>[4x]GMTDIPDRKEAVISLWPEFAKAIVSGKKTVEFRRRIPLPALSARIWIYATRPVKSVIGFAYLEAIVQGDVNTLWSRYGREAFLSEQQYRDYFEGTEKATAFLLRDHQPIRPINLDQ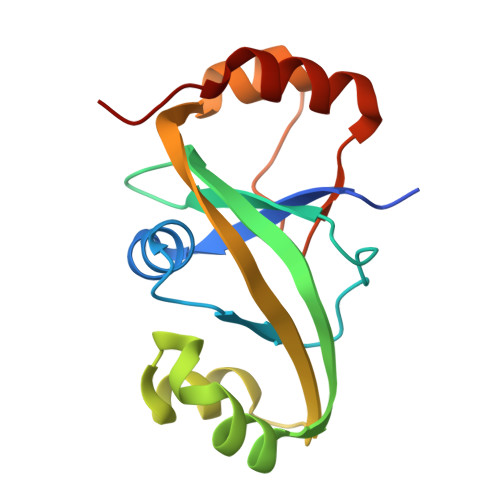LKEIRANFQPPQSLTWLRKEETQKLVSLTSQVE> KVSVNDIMVPRNEIVGIDINDDWKSIVRQLTHSPHGRIVLYRDSLDDAISMLRVREAYRLMTEKKEFTKEIMLRA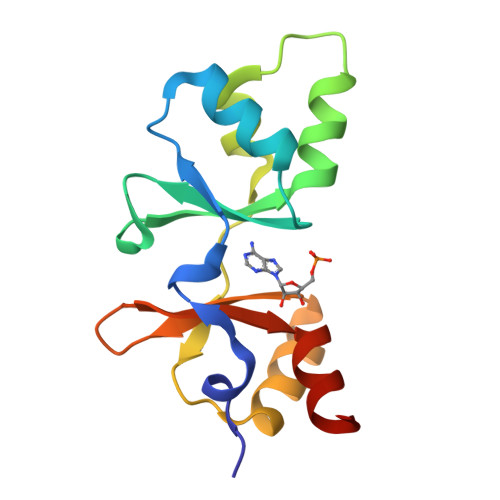ADEIYFVPEGTPLSTQLVKFQRNKKKVGLVVDEYGDIQGLVTVEDILEEIVGDFT Noroviruses have been identified as major causative agents of acute nonbacterial gastroenteritis in humans. Histo‐blood group antigens (HBGAs) are thought to play a major role among the host cellular factors influencing norovirus infection. Genogroup I, genotype 9 (GI.9) is the most recently identified genotype within genogroup I, whose representative strain is the Vancouver 730 norovirus. We determined the crystal structures of the protruding domain of the GI.9 capsid protein in the presence or absence of Lewis antigens.

In this study, we demonstrate that the GI.9 norovirus preferentially binds Lewis antigens over blood group A, B, and H antigens, as revealed by an HBGA binding assay using virus‐like particles. Our analysis demonstrated that Lewis fucose (α1–3/4 fucose) represents a key moiety for the GI.9 protein–HBGA interaction, thus suggesting that Lewis antigens might play a critical role during norovirus infection.

>QKTKQFSVPNLPLNVMSNSRVPSLLNAMVVSPDQAQVVQFQNGRCTLDGQMLGTTTVSASCVARFRGKTFQAPDNRLGINLAEISGEPYHAFESPAPLGFPDFGDGDWHVTATKVTPSQLEANDPVVVGNVQPYNPQFAPHLGTLVVENPTPDQVATGTDLLFNITWLSNRANNRFNPWVIPNYGSTLTEAAQLAPSIFPPGFGETIVYFNSTFPAVGATTHAAIPCLLPQEFVAHFVNEQAPIRGEAALLHYIDPDTHRNLGEFKIYPEGFVTCVPNVGGTGPQSLPTNGVFVFVSWVSRYYQLKPVGTAG[2x]>DITVYNG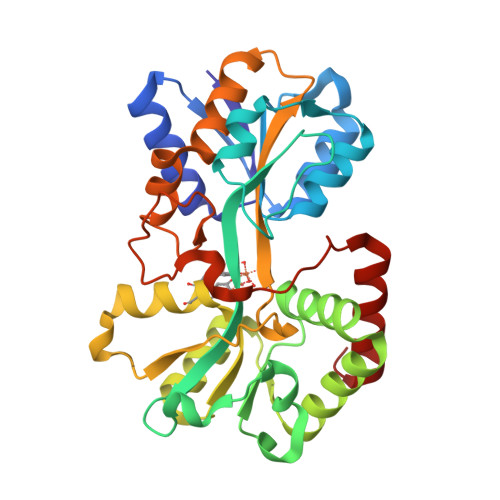QHKEAAQAVADAFTRATGIKVKLNSAKGDQLAGQIKEEGSRSPADVFYSEQIPALATLSAANLLEPLPASTINETRGKGVPVAAKKDWVALSGRSRVVVYDTRKLSEKDLEKSVLNYATPKWKNRIGYVPTSGAFLEQIVAIVKLKGEAAALKWLKGLKEYGKPYAKNSVALQAVENGEIDAALINNYYWHAFAREKGVQNVHTRLNFVRHRDPGALVTYSGAAVLKSSQNKDEAKKFVAFLAGKEGQRALTAVRAEYPLNPHVVSTFNLEPIAKLEAPQVSATTVSEKEHATRLLEQAGMK[9x]>AAASMSALITENMHMKLYMEGTVNNHHFKCTSEGEGKPYEGTQTMRIKVVEGGPLPFAFDILATSFMYGSKTFINHTQGIPDFFKQSFPEGFTWERVTTYEDGGVLTATQDTSLQDGCLIYNVKIRGVNFPSNGPVMQKKTLGWEASTEMLYPADGGLEGRADMALKLVGGGHLICNLKTTYRSKKPAKNLKMPGVYYVDRRLERIKEADKETYVEQHEVAVA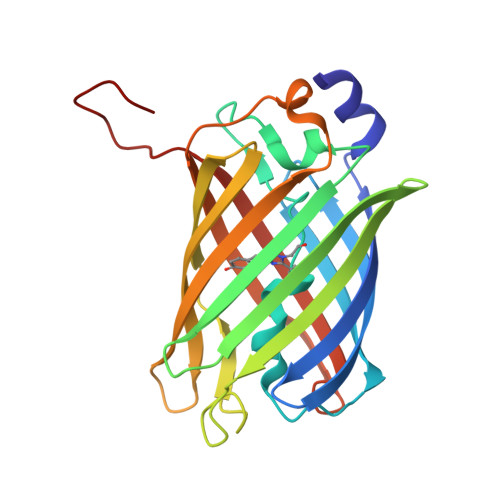RYCDLPSKLAHK[4x]> AMENKIEVNNKDEMNRWFEEFKKGNGLVDTFTNSYSFCESVPNLDRFVFQMASATDDAQKDSIYASALVEATKFCAPIYECAWVSSTGIVKKGLEWFEKNAGTIKSWDESYTELKVDVPKIEQLTGYQQAALKWRKDIGFRVNANTAALSNKVLAEYKVPGEIVMSVKEMLSDMIRRRNLILNRGGDENPRGPVSHEHVDWCREFVKGKYIMAFNPPWGDINKSGRSGIALVATGLAKLAETEGKGIFDEAKKTVEALNGYLDKHKDEVDRASADSMITNLLKHIAKAQELYKNSSALRAQSAQIDTAFSSYYWLYKAGVTPETFPTVSQFLFELGKQPRGTKKMKKALLSTPMKWGKKLYELFADDSFQQNRIYMHPAVLTAGRISEMGVCFGTIPVANPDDAAQGSGHTKSILNLRTNTE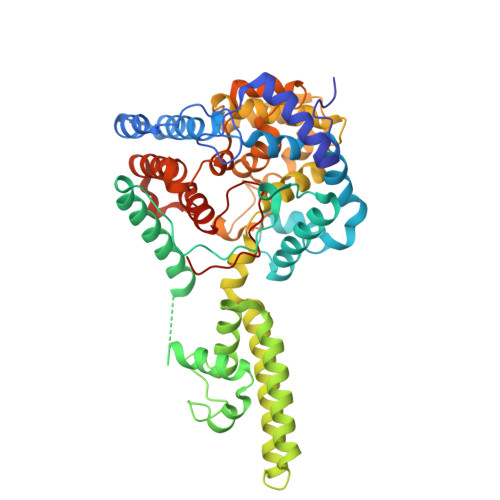TNNPCAKTIVKLFEVQKTGFNIQDMDIVASEHLLHQSLVGKQSPFQNAYNVKGNATSANII>[6x]MVQAVAVLKGDAGVSGVVKFEQASESEPTTVSYEIAGNSPNAERGFHIHEFGDATNGCVSAGPHFNPFKKTHGAPTDEVRHVGDMGNVKTDENGVAKGSFKDSLIKLI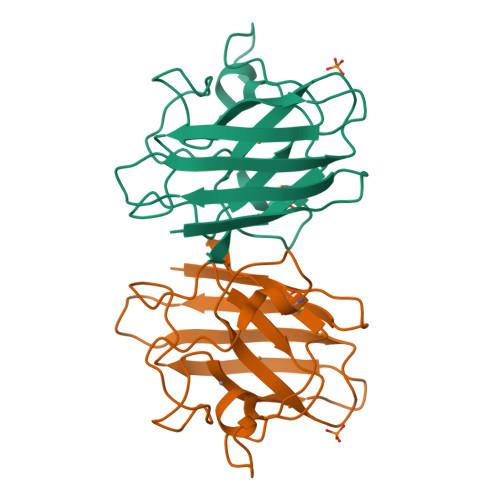GPTSVVGRSVVIHAGQDDLGKGDTEESLKTGNAGPRPACGVIGLTN> MAHPGRTGYDNREIVMKYIHYKLSQRGYEWDAGDDVEENRTEAPEGTESEVVHLTLRQAGDDFSRRYRRDFAEMSSQLHLTPFTARGRFATVVEELFRDGVNWGRIVAFFEFGGVMCVESVNREMSPLVDNIALWMTE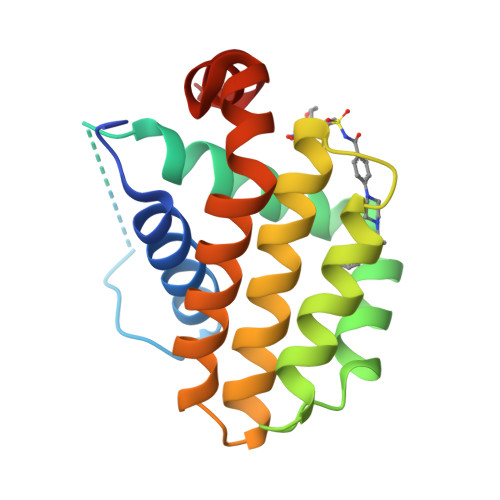YLNRHLHTWIQDNGGWDAFVELYGPSMR>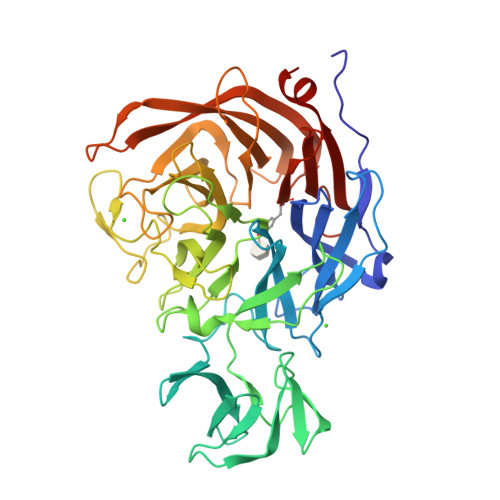[2x]VEGAVKTEPVDLFHPGFLNSSNYRIPALFKTKEGTLIASIDARRHGGADAPNNDIDTAVRRSEDGGKTWDEGQIIMDYPDKSSVIDTTLIQDDETGRIFLLVTHFPSKYGFWNAGLGSGFKNIDGKEYLCLYDSSGKEFTVRENVVYDKDSNKTEYTTNALGDLFKNGTKIDNINSSTAPLKAKGTSYINLVYSDDDGKTWSEPQNINFQVKKDWMKFLGIAPGRGIQIKNGEHKGRIVVPVYYTNEKGKQSSAVIYSDDSGKNWTIGESPNDNRKLENGKIINSKTLSDDAPQLTECQVVEMPNGQLKLFMRNLSGYLNIATSFDGGATWDETVEKDTNVLEPYCQLSVINYSQKVDGKDAVIFSNPNARSRSNGTVRIGLINQVGTYENGEPKYEFDWKYNKLVKPGYYAYSCLTELSNGNIGLLYEGTPSEEMSYIEMNLKYLESGANK>[2x]MYTLNWQPPYDWSWMLGFLAARAVSSVETVADSYYARSLAVGEYRGVVTAIPDIARHTL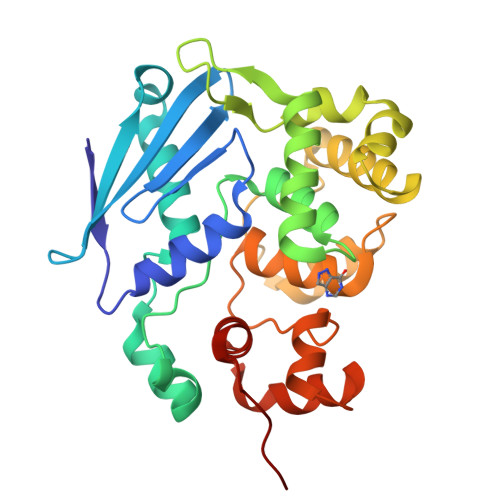HINLSAGLEPVAAECLAKMSRLFDLQCNPQIVNGALGRLGAARPGLRLPGCVDAFEQGVRAILGQLVSVAMAAKLTARVAQLYGERLDDFPEYICFPTPQRLAAADPQALKALGMPLKRAEALIHLANAALEGTLPMTIPGDVEQAMKTLQTFPGIGRWTANYFALRGWQAKDVFLPDDYLIKQRFPGMTPAQIRRYAERWKPWRSYALLHIWYTEGWQPDEA> NLFQFAKMINGKLGAFSVWNYISYGCYCGWGGQGTP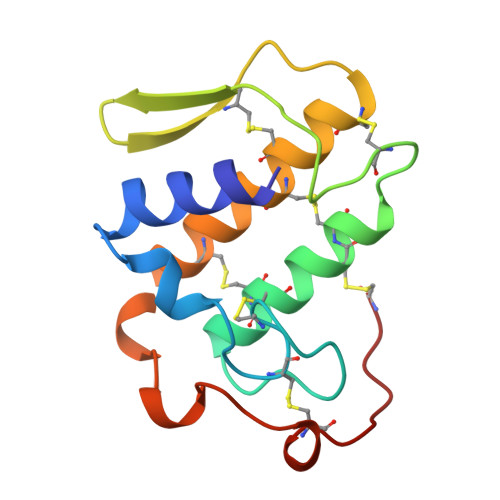KDATDRCCFVHDCCYGRVRGCNPKLAIYYYSFKKGNIVCGKNNGCLRDICECDRVAANCFHQNKNTYNANYKFLSSSRCRQTGEKC> AHHHHHHGSVKVKVKYFARFRQLAGVDEE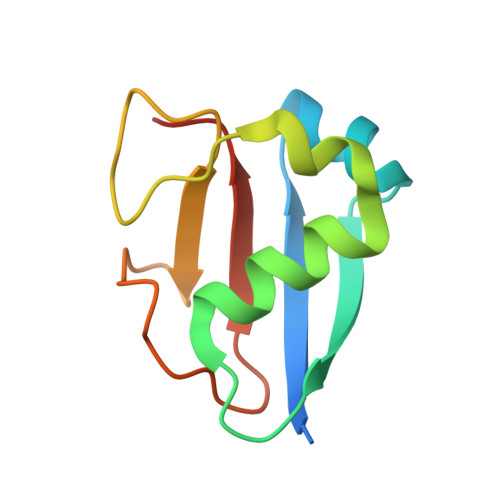EIELPEGARVRDLIEEIKKRHEKFKEEVFGEGYDEDADVNIAVNGRYVSWDEELKDGDVVGVFPPVSGG>[2x]SVPKTGDSLAMARRLARSVRRLTRRRAHRLLRTRRLLKREGVLQAANFDENGLIKSLPNTPWQLRAAALDRKLT;>[4x]SMASKNNIFNK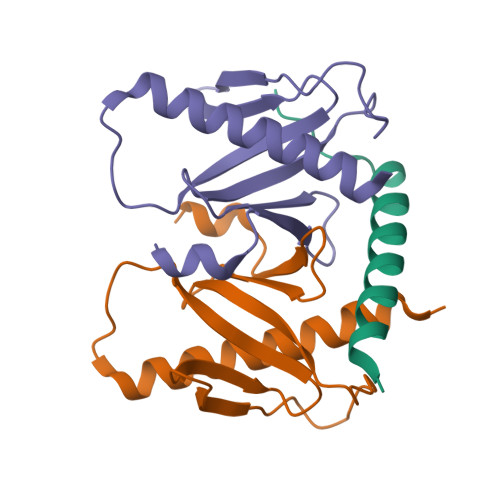YPTIIHGEARGENDEFVVHTRYPRFLARKSFDDNFTGEMPAKPVNGELGQIGEPRRLAYDSRLGLWLSDFIMLDNNKPKNMEDWLGQLKAACDRIAADDLMLNEDAADLEGWDD PARP4 is an ADP-ribosyltransferase that resides within the vault ribonucleoprotein organelle. PARP4 is an ADP-ribosyltransferase that uses NAD+ as a substrate to synthesize ADP-ribose modifications on molecules. The PARP1-homology region of PARP4 includes a BRCT fold, a WGR domain, and the catalytic (CAT) domain. However, PARP3 and PARP4 contain the catalytic triad H-Y-E but are considered MARylation enzymes, indicating that other structural features are important determinants of catalytic output.

We also determined structures of the PARP4 ART domain alone (CATΔHD), which provided higher-resolution insights into the active site configuration that gives rise to PARP4 mono(ADP-ribosylation) activity. The HD was replaced with an 8-residue linker (GSGSGSGG) connecting L282 to S365. CATΔHD crystallized in complex with EB47, and in complex with NADH, the non-hydrolysable reduced form of NAD+. The CATΔHD/EB47 crystals diffracted to 3.0 Å and belonged to space group C2221 with three PARP4 molecules in the asymmetric unit. Again, only two PARP4 molecules contained EB47 in the active site, due to a crystal contact in the active site of the third PARP4 molecule. Structure refinement yielded a crystallographic R/RFREE of 0.203/0.248. An alignment of all of the ART structures determined in this study did not provide any evidence of flexibility in the acceptor site region of PARP4. This analysis suggests that the positioning of residues surrounding the acceptor site region are largely static. We have also determined crystal structures of the PARP4 ART fold that illustrate that multiple alterations to the ‘acceptor’ site have rendered PARP4 incapable of PARylation, despite the H-Y-E motif.

>[3x]SSEQLQALLLEEVMNSSTLSQEVSDLVEMIWAEALGHLEHMLGSGSGSGGSKPNPPSLAKYRALRCKIEHVEQNTEEFLRVRKEVLQNHHSKSPVDVLQIFRVGRVNETTEFLSKLGNVRPLLHGSPVQNIVGILCRGLLLPKVVEDRGVQRTDVGNLGSGIYFSDSLSTSIKYSHPGETDGTRLLLICDVALGKCMDLHEKDFSLTEAPPGYDSVHGVSQTASVTTDFEDDEFVVYKTNQVKMKYIIKFSMPGDQIKD[oxidanyl-[(2S,3R,5S,6S)-4-phenylmethoxy-2,3,5,6-tetraphosphonooxy-cyclohexyl]oxy-phosphoryl]methylphosphonic 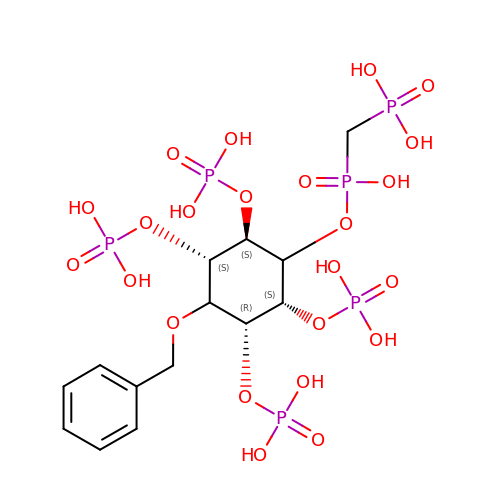acid | C14 H26 O23 P6 | WTIJGFYHWWTXHU-BUCHIQEDSA-N> AKWVYKFEEGNASMRNLLGGAGCNLAEMTILGMPIPQGFTVTTEACTEYYNSG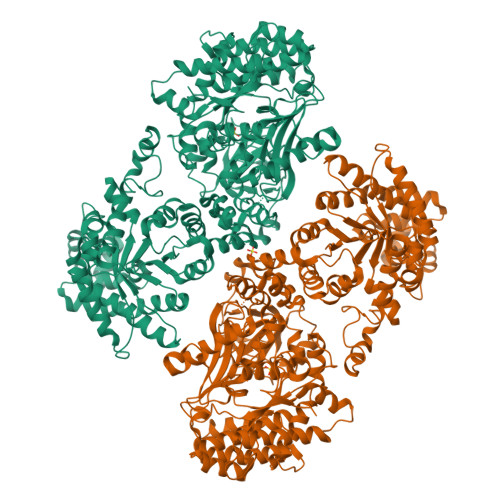KQITQEIQDQIFEAITWLEELNGKKFGDTEDPLLVSVRSGARASMPGMMDTILNLGLNDVAVEGFAKKTGNPRFAYDSYRRFIQMYSDVVMEVPKSHFEKIIDAMKEEKGVHFDTDLTADDLKELAEKFKAVYKEAMNGEEFPQEPKDQLMGAVKAVFRSWDNPRAIVYRRMNDIPGDWGTAVNVQTMVFGNKGETSGTGVAFTRNPSTGEKGIYGEYLINAQGEDVVAGVRTPQPITQLENDMPDCYKQFMDLAMKLEKHFRDMQDMEFTIEEGKLYFLQTRNGKRTAPAALQIACDLVDEGMITEEEAVVRIEAKSLDQLLHPTFNPAALKAGEVIGSALPASPGAAAGKVYFTADEAKAAHEKGERVILVRLETSPEDIEGMHAAEGILTVRGGMTSHAAVVARGMGTCCVSGCGEIKINEEAKTFELGGHTFAEGDYISLDGSTGKIYKGDIETQEASVSGSFERIMVWADKFRTLKVRTNADTPEDTLNAVKLGAEGIGLCRTEHMFFEADRIMKIRKMILSDSVEAREEALNELIPFQKGDFKAMYKALEGRPMTVRYLDPPLHEFVPHTEEEQAELAKNMGLTLAEVKAKVDELHEFNPMMGHRGCRLAVTYPEIAKMQTRAVMEAAIEVKEETGIDIVPEIMIPLVGEKKELKFVKDVVVEVAEQVKKEKGSDMQYHIGTMIEIPRAALTADAIAEEAEFFSFGTNDLTQMTFGFSRDDAGKFLDSYYKAKIYESDPFARLDQTGVGQLVEMAVKKGRQTRPGLKCGICGEHGGDPSSVEFCHKVGLNYVSCSPFRVPIARLAAAQAALNNK Here, we investigated the biochemical, structural, and dynamic properties of the enzyme complex responsible for vitamin B6 (pyridoxal 5-phosphate, PLP) biosynthesis in S. aureus, which comprises enzymes SaPdx1 and SaPdx2. A multimeric assembly of two enzymes, Pdx1 and Pdx2, synthesizes pyridoxal 5-phosphate (PLP), the active form of vitamin B6, as well as its vitamers. Pdx2 has glutaminase activity, converting L-glutamine into L-glutamate and an ammonia molecule. The latter is delivered to Pdx1, which synthesizes PLP using ammonia, ribose 5-phosphate (R5P), and glyceraldehyde 3-phosphate (G3P).

Crystals of SaPdx1 were obtained, and a dataset was recorded at the MANACA beamline at the Brazilian Sirius light source. The structure was solved by molecular replacement with an AF2 model and refined to 3.0 Å resolution. The asymmetric unit was composed of two SaPdx1 monomers, but the H32 crystal symmetry readily revealed the dodecameric structure of the PLP synthase enzyme. The dodecamer forms a cylindrical quaternary structure with an opening diameter of approximately 52 Å and a lateral height of approximately 84 Å. Each monomer is folded as a slightly distorted eight-stranded TIM-barrel with the top of the barrel pointing toward the internal aperture of the cylindrical quaternary structure. The experimental electron density allowed the modeling of residues 17 to 272 out of the 297 residues of the enzyme, with a missing region including seven residues in the ‹2′ region. Two electron densities were identified in the P2 phosphate binding site, and the densities were modeled as phosphate molecules interacting with R138 and R139 from the LGEAxRRI sequence motif. Additionally, an ethylene glycol (EDO) molecule was observed to bind to the active site of SaPdx1 close to the catalytic lysine. For one of the monomers in the asymmetric unit (chain B), a hydrogen bond was clearly formed between K82 and the ethylene glycol molecule.

>[2x]GAMSKIIGSDRVKRGMAEMQKGGVIMDVVNAEQARIAEEAGAVAVMALERVPSDIRAAGGVARMANPKIVEEVMNAVSIPVMAKARIGHITEARVLEAMGVDYIDESEVLTPADEEYHLRKDQFTVPFVCGCRNLGEAARRIGEGAAMLRTKGEPGTGNIVEAVRHMRQVNSEVSRLTVMNDDEIMTFAKDIGAPYEILKQIKDNGRLPVVNFAAGGVATPQDAALMMELGADGVFVGSGIFKSEDPEKFAKAIVQATTHYQDYELIGRLASELGTAMKGLDINQLSLEERMQERGW> TTGHSYEKYNNWETIEAWTEQVA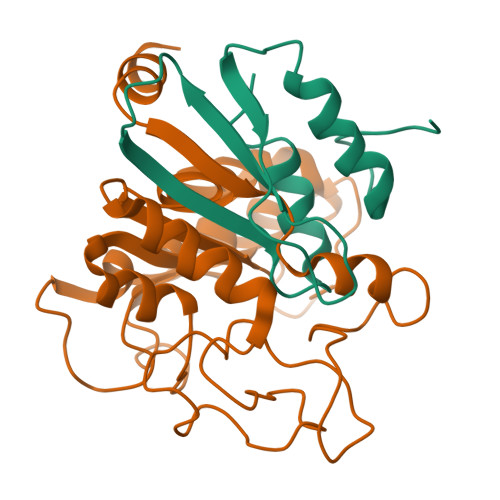SENPDLISRSAIGTTFLGNTIYLLKVGKPGSNKPAVFMDCGFHAREWISPAFCQWFVRE;> EIHMTEFLDKLDFYVLPVVNIDGYIYTWTTNRMWRKTRSTRAGSSCTGTDLNRNFDAGWCSIGASNNPCSETYCGSAAESEKESKAVADFIRNHLSSIKAYLTIHSYSQMMLYPYSYDYKLPKNNVELNTLAKGAVKKLASLHGTTYSYGPGATTIYPASGGSDDWAYDQGIKYSFTFELRDKGRYGFVLPESQIQPTCEETMLAIKYVTSYVLEHL>HHHHMRVSFMVAMDENRVIGKDNNLPWRLPSELQYVKKTTMGHPLIMGRKNYE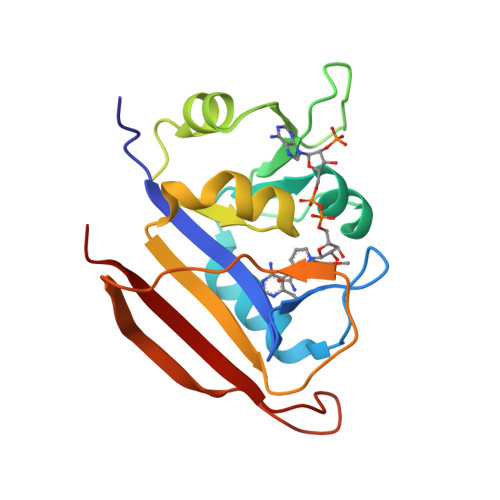AIGRPLPGRRNIIVTRNEGYHVEGCEVAHSVEEVFELCKNEEEIFIFGGAQIYDLFLPYVDKLYITKIHHAFEGDTFFPEMDMTNWKEVFVEKGLTDEKNPYTYYYHVYEKQQ[2x]>MSLLNNKAGVISRLADFLGFRPKTGDIDVMNRQSVGSVTISQLAKGFYEPNIESAINDVHNFSIKDVGTIITNKTGVSPEGVSQTDYWAFSGTVTDDSLPPGSPITVLVFGLPVSATTGMTAIEFVAKVRVALQEAIASFTAINSYKDHPTDGSKLEVTYL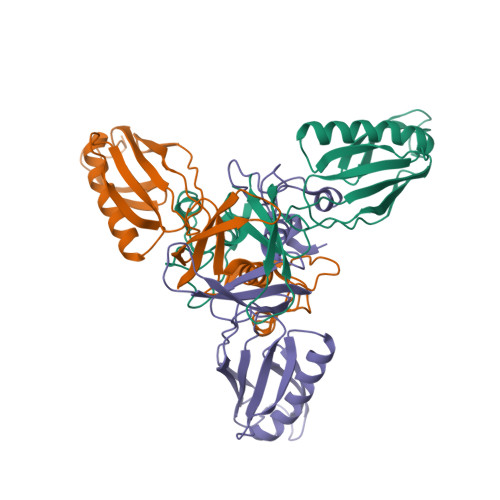DNQKHVLSTYSTYGITISQEIISESKPGYGTWNLLGAQTVTLDNQQTPTVFYHFERTA[3x]>[10x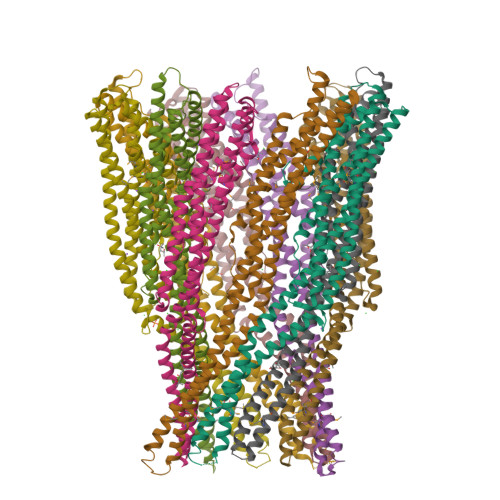]MTNATTITMDQGMANQASQAMQIQTYCNSVKQQVPVDFSQFPNLKDNQTQINQGLDLAKGHADLYLNTIQPQIITNISNISNYFALQNAIPAVLPPGSTKAQWLRQLSVIKEQATEYQRLSSDTRLVIVNLNNNLITDSSNFQGIVVNLNSKVQGDNGVLAQLNGDIDKVNAAIDGAIAGIVAGGLLVIGGAFVTAIGAVADFVTAGTSTPVVIGGVAMMVAGAGGITAGAIVLHNSLGARQDLYQKRSSLNSEVLIATQIGNGYKGLQVQAQNAVTAATQMSNAWDSLTSDLGSLITDLDKGITSGDDIRQLWLTAADTTVKTVLTDVTTIKAQIAGVSPLQVPQTDTIANFVARLAALEHHHHHH> TGGVQTVTLIPGDGIGPEISAAVMKIFDAAKAPIQWEERNVTAIQGPGGKWMIPSEAKESMDKNKMGLKGPLKTPIAAGHPSMNLLLRKTFDLYANVRPCVSIEGYKTPYTDVNIVTIRENTEGEYSGIEHVIVDGVVASIKLITEGASKRIAEFAFEYARNNHRSNVTAVHKANIMRMSDGLFLQKCREVAESCKDIKFNEMYLDTVCL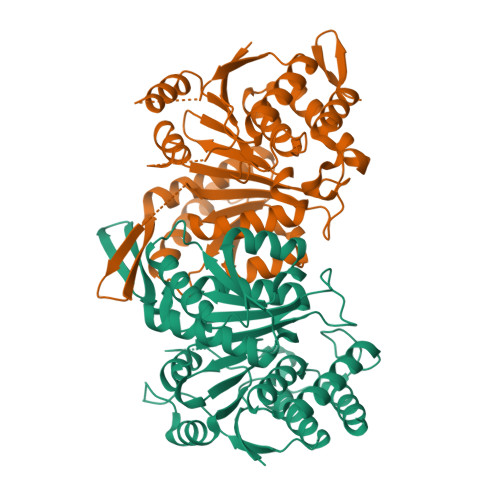NMVQDPSQFDVLVMPNLYGDILSDLCAGLIGGLGVTPSGNIGANGVAIFESVHGTAPDIAGKDMANPTALLLSAVMMLRHMGLFDHAARIEAACFATIKDGKSLTKDLGGNAKCSDFTEEICRRVKDLD;> FSEQTIPPSAKYGGRHTVTMIPGDGIGPELMLHVKSVFRHACVPVDFEEVHVSSNADEEDIRNAIMAIRRNRVALKGNIETNHNLPPSHKSRNNILRTSLDLYANVIHCKSLPGVVTRHKDIDILIVRENTEGEYSSLEHESVAGVVESLKIITKAKSLRIAEYAFKLAQESGRKKVTAVHKANIMKLGDGLFLQCCREVAARYPQITFENMIVDNTTMQLVSRPQQFDVMVMPNLYGNIVNNVCAGLVGGPGLVAGANYGHVYAVFETATRNTGKSIANKNIANPTATLLASCMMLDHLKLHSYATSIRKAVLASMDNENMHTPDIGGQGTTSEAIQDVIRHIRVINGRAVEA> LPGECSVNVIPKKNLDKAKFFSGTWYETHYLDMDPQATEKFCFSFAPRESGGTVKEALYHFNVDSKVSFYNTGTGPLESNGAKYTAKFNTVDKKGKEIKPADEKYSYTVTVIEAAKQSALIHICLQEDGKDIGDLYSVLNRNKNALPNKKIKKALNKVSLVLTKFVVTKDLDCKYDDKFLSSW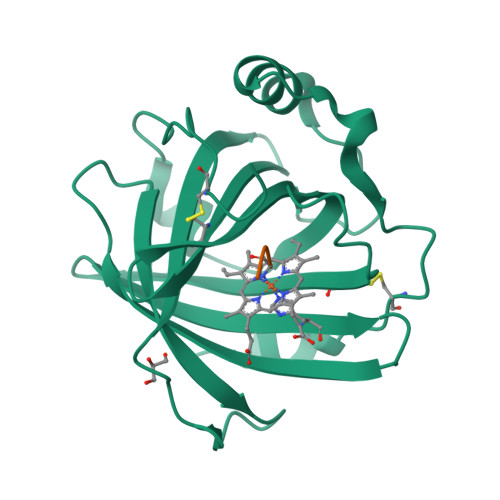QK;> GGG EgtD, an S-adenosylmethionine-dependent methyltransferase (AdoMet), catalyzes the trimethylation of L-Histidine to initiate EGT biosynthesis and this reaction has been shown to be essential for EGT production in mycobacteria and for long-term infection of murine macrophages by M. tb. Synthesis of EGT by Mycobacterium tuberculosis (M. tb) is critical for maintaining bioenergetic homeostasis and protecting the bacterium from alkylating agents, oxidative stress, and anti-tubercular drugs. Multiple X-ray crystal structures of Mycolicibacterium smegmatis EgtD show that EgtD possesses a Histidine binding domain and a Rossmann-fold domain, which affords ordered substrate binding of L-Histidine and AdoMet, respectively. In this work, library screening and structure-guided strategies identified multiple classes of M. tb EgtD inhibitors that bind in various regions of the enzyme active site.

The obtained crystals were subjected to X-ray diffraction experiments and X-ray crystal structures were obtained for M. tb EgtD with HD2, HD3, and HD6. The chemical structure of HD6 is very similar to that of HD2, so the interactions between EgtD and HD6 are nearly identical to those with HD2. The only difference observed is a rotamer change in the side chain of Glu282 resulting in slight reorientation of the carboxylate moiety. However, the presence of a hydrogen atom on the α-amino moiety of HD6 now affords a bidentate interaction between Asn166 and HD6, which is more similar to the interaction between EgtD and the L-Histidine substrate. First, HD2, HD3, and HD6 most closely resemble a Histidine amino acid as they all possess α-amino and α-carboxyl moieties, but the α-amino group is elaborated with a variety of chemical linkages. The reason for the 1.5–2.5-fold decrease in the HD6 inhibitory activity versus HD2 and HD3 is less clear but is likely derived from steric hindrance between the cyclopentene and the narrow constriction separating the Histidine and AdoMet binding sites. The observed crystal structures of EgtD-Histidine-/Histamine-derivative complexes, consistent with the changes observed upon L-Histidine binding to EgtD, exhibit only minor variation in the side chain rotamers of residues forming the substrate binding sites.

> GPVSVANHLGEDAGHLALRRDVYSGLQKTPKSLPPKWFYDTVGSELFDQITRLPEYYPTRAEAEILRARSAEVASACRADTLVELGSGTSEKTRMLLDALRHRGSLRRFVPFDVDASVLSATATAIQREYSGVEINAVCGDFEEHLTEIPRGGRRLFVFLGSTIGNLTPGPRAQFLTALAGVMRPGDSLLLGTDLVKDAARLVRAYDDPGGVTAQFNRNVLAVINRELEADFDVDAFQHVARWNSAEERIEMWLRADGRQRVRVGALDLTVDFDAGEEMLTEVSCKFRPQAVGAELAAAGLHRIRWWTDEAGDFGLSLAAK4-methyl-5-[2-(phosphonooxy)ethyl]-1,3-thiazole-2-carboxylic acid | C7 H10 N O6 P S | 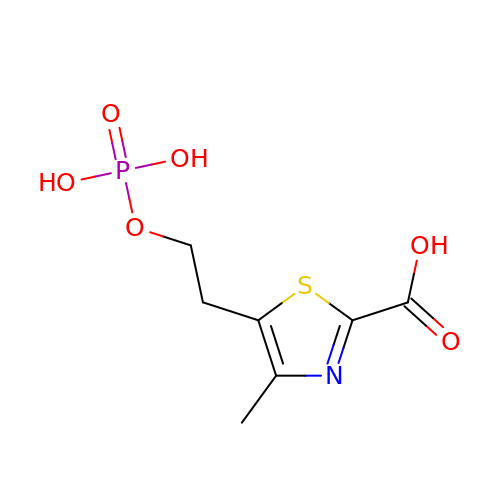XWECMAHAKFWYNV-UHFFFAOYSA-N>MVFEENSDEVRVITLDHPNKHNPFSRTLETSVKDALARANADDSVRAVVVYGGAERSFSAGGDFNEVKQLSRSEDIEEWIDRVIDLYQAVLNVNKPTIAAVDGYAIGMGFQFALMFDQRLMASTANFVMPELKHGIGCSVGAAILGFTHGFSTMQEI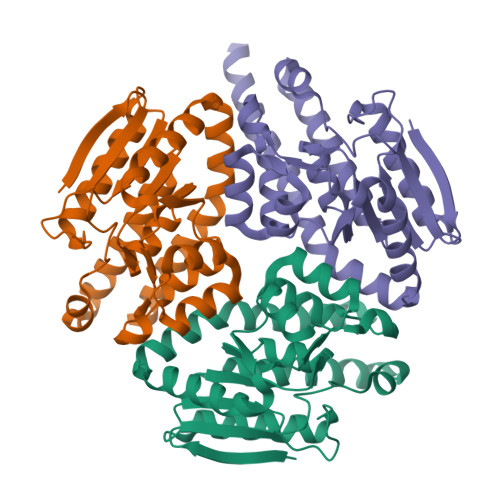IYQCQSLDAPRCVDYRLVNQVVESSALLDAAITQAHVMASYPASAFINTKRAVNKPFIHLLEQTRDASKAVHKAAFQARDAQGHFKNVLGKKY[9x]>[2x]MVEINNQRKAFLDMLAWSEGTDN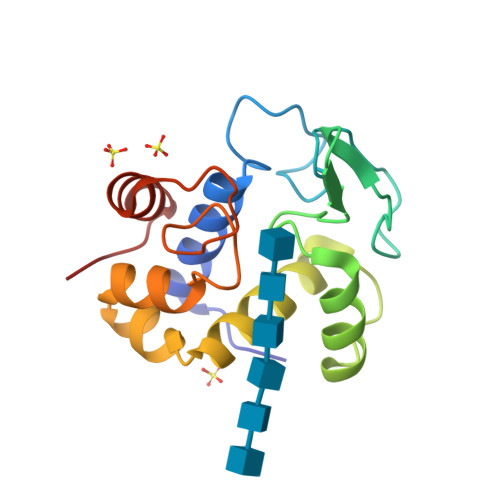GRQKTRNHGYDVIVGGELFTDYSDHPRKLVTLNPKLKSTGAGRYQLLSRWWDAYRKQLGLKDFSPKSQDAVALQQIKERGALPMIDRGDIRQAIDRCSNIWASLPGAGYGQFEHKADSLIAKFKEAGGTVR>[3x]MGQIFSRSASPIPRPPRGLAAHHWLNFLQAAYRLEPGPSSYDFHQLKKFLKIALETPARICPINYSLLASLLPKGYPGRVNEILHILIQTQAQIPSRPAPPPPSSPTHDPPDSDPQIPPPYVEPTAPQVLPVMHPHGAPPNHRPWQMKDLQAIKQEVSQAAPGSPQFMQTIRLAVQQFDPTAKDLQDLLQYLCSSLVASLHHQQLDSLISEAETRGITGYNPLAGPLRVQANNPQQQGLRREYQQLWLAAFAALPGSAKDPSWASILQGLEEPYHAFVERLNIALDNGLPEGTPKDPILRSLAYSNANKECQKLLQARGHTNSPLGDMLRACQTWTPKDKTKVLVVQPKKPPPNQPCFRCGKAGHWSRDCTQPRPPPGPCPLCQDPTHWKRDCPRLKPTIPEPEPEEDALLLDLPADIPHPKNSIGGEV

The retroviral structural protein Gag forms the immature protein shell of nascent virus particles4. All retroviral Gag proteins contain three canonical domains: matrix (MA), capsid (CA), consisting of independently folded N-terminal (CA-NTD) and C-terminal (CA-CTD) domains, and nucleocapsid (NC). During immature virus particle formation, these domains function in membrane binding, viral lattice self-assembly and viral genomic RNA (vgRNA) packaging, respectively. Our results show that HTLV-1 uses a distinct CA-NTD arrangement to form the immature Gag lattice and that, in contrast to other retroviral structures, the CA-NTD is the key determinant of immature HTLV-1 assembly.

To gain insight into the immature architecture of HTLV-1, we used cryo-ET to visualize mammalian cell-derived Gag-based VLPs. The CA layer exhibited a regular organization; hence, we used subtomogram averaging to obtain higher-resolution information for this layer. However, to account for the observed heterogeneity of HTLV-1 Gag VLP shapes, we applied local C2 symmetry during subtomogram averaging. The resulting maps had a CA-CTD layer that was resolved to a lower resolution than the CA-NTD layer, which we predict is because of heterogeneity caused by flexibility of the CA-CTD. In contrast, the CA-NTD did not show increased heterogeneity. Therefore, we used both domains as independent species in a multiparticle refinement using the software M34. This approach yielded 5.9-Å and 6.2-Å resolution maps of the CA-NTD and CA-CTD layers, respectively. The CA-NTD establishes lateral interactions that form two basic building blocks shaping the lattice: a CA-NTD trimer and a CA-NTD hexamer. The trimer is formed by interactions spanning residues in helices 4 and 5. Similarly, the hexamerization interface involves helices 1, 2 and 3 of two neighboring monomers (annotated I and I′ in Fig. 1e,h).> XT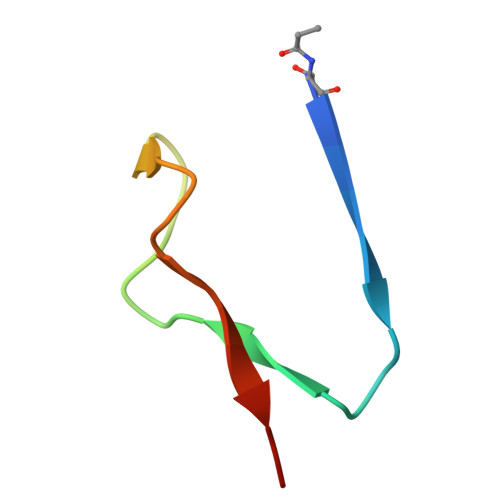VINLFAPGKVNLVEQLESLSVTKIGQPLAVSTET>[6x]MASHHHHHHDYDGATTENLYFQGSMDVVDPDIFNRDPRDHYDLLQRLGGGT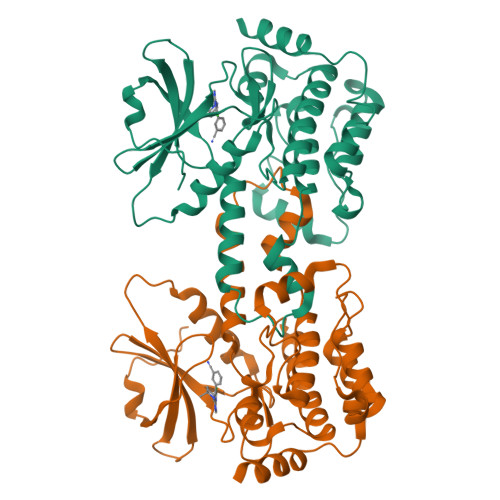YGEVFKARDKVSGDLVALKMVKMEPDDDVSTLQKEILILKTCRHANIVAYHGSYLWLQKLWICMEFCGAGSLQDIYQVTGSLSELQISYVCREVLQGLAYLHSQKKIHRDIKGANILINDAGEVRLADFGISAQIGAELARRLEFIGTPYWMAPEVAAVALKGGYNELCDIWSLGITAIELAELQPPLFDVHPLRVLFLMTKSGYQPPRLKEKGKWSAAFHNFIKVTLTKSPKKRPSATKMLSHQLVSQPGLNRGLILDLLDKLKNPGKGPSIGDIEDEE The genome of C. divulgatum encodes three GH1 enzyme candidates, from which CIB12 and CIB13 were heterologously expressed and characterized. Purified CIB12 and CIB13 were crystallized using the sitting-drop vapor diffusion method, and their crystal structures were determined to 2.55 Å and 2.22 Å resolution, respectively, by molecular replacement (see the section “Materials and methods” for details). Both structures revealed a classical (β/α)8 TIM-barrel fold with a spherical shape, which is typical for GH1 enzymes and is one of the most common protein folds. In the retaining catalytic mechanism of GH1 hydrolases, one of the two glutamates acts as an acid/base catalyst (Glu204 in CIB12 and CIB13) and the other acts as a nucleophile (Glu388 in CIB12 and Glu385 in CIB13). In this work, two representatives of glycosidases of GH1 family from C. divulgatum were characterized. Both CIB12 and CIB13 were active against cellobiose and lactose but showed substrate preference to cellobiose, and therefore were identified as cellobiohydrolases, EC 3.2.1.21.

In addition, the CIB12 structure contains two small antiparallel and one parallel β-sheets and six short α-helices, whereas CIB13 has four antiparallel β-sheets with two β-strands each and four α-helices outside the barrel structure. Both CIB12 and CIB13 structures revealed the presence of two protomers per asymmetric unit forming a dimer with interacting residues located primarily on two C-terminal α-helices, one side β-strand, and connecting loops. The cleavage of the glycosidic bond involves the formation of a covalent glucosyl-enzyme intermediate, which is then deglycosylated in a hydrolysis reaction via the attack of a water molecule producing the free enzyme and glucose. Both active sites show the presence of an additional area of electron density in each protomer located near the catalytic glutamates: Glu204 (3.9 Å) and Glu388 (2.8 Å) in CIB12 and Glu204 (3.5 Å) and Glu385 (2.8 Å) in CIB13. In CIB12, this density was interpreted as glycerol (two molecules in the CIB12 dimer), whereas the CIB13 dimer contained one molecule of glycerol in one protomer and one molecule of tris(hydroxymethyl)aminomethane (Tris) in the second protomer. The glycerol molecule in the CIB12 active site was also positioned close to the side chains of conserved His148 (3.1 Å), Trp149 (4.5 Å), Tyr321 (3.9 Å), Trp426 (4.1 Å), Glu433 (2.9 Å), and Trp434 (3.4 Å). Additionally, both active sites contained several aromatic and charged residues, which might contribute to substrate binding including Gln16, Trp30, Asn203, Glu207, Tyr341, Trp362, and Phe442 in CIB12 and Gln16, Trp30, Asn203, Phe340, Met357, and Trp359 in CIB13. The crystal structure of CIB12 also revealed the presence of the disulfide bond Cys172–Cys212 located near the active site, which is not conserved in CIB13 and might contribute to a higher thermotolerance of CIB12 activity compared to CIB13.

>MFPKNFKFGFSEAGFQFEMGVSDIDTNTDWYKWSHDSENIKNHIVSGDRPEEGVGYWDLYPKDHDLAEYIGMNAARIGIEWSRIFPVSTERVTVEVIEENGDILEIKITEKTIKELDLLSDKNAMQHYTNIFNDIKKRGWFLVINLFHWSLPLWINDPSNRNSEKDNALGNCMNRSSVIEFVKYAAYISYYFGSIADRFATMNEPNEVFKTCSEDKRVESYHIRMKWFVEAHARSYDAMKQFTNRQIGVIYANGDVQSFENKDPKLKEEVEYEQRYSFFDALIHGDVHWYVGACRKTNHVHGKSIRPDLSNRIDWIGVNYYSRNVVKRKEDGYENVRGLGYDTGWVSYEKSLDGRSVSETGWEIYPEGIYNIVMSYHKRYELPMMITENGMADDNDRFRPRYLVSHLKNLERAINDGAKVDGYLHWALTDNFEWGSGFSKKFGLIKVDYKTKKRYLRPSALIMKEITKHNGIPEELEWLGEDKF[2x]>[2x]GSHMQNTFLDTIATRFDGTHSNFVLGNAQANGNPIVYCSDGFVDLTGYSRAQIMQKGCSCHFLYGPDTKEEHKQQIEKSLSNKMELKLEVIFYKKEGAPFWC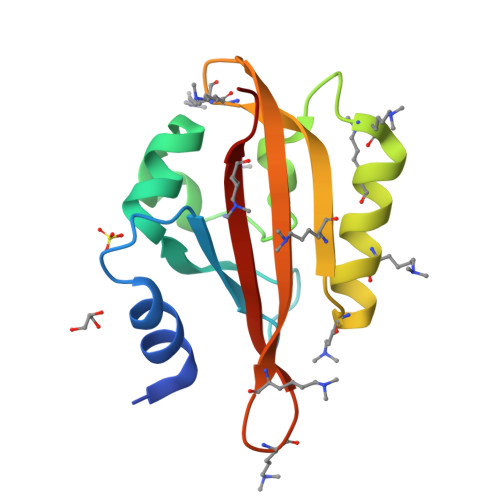LFDIVPIKNEKRDVVLFLASHKDITHTK> MLFTVTAPKEVYTVDVGSSVSLECDFDRRECTELEGIRASLQKVENDTSLQSERATLLEEQLPLGKALFHIPSVQVRDSGQYRCLVICGAAW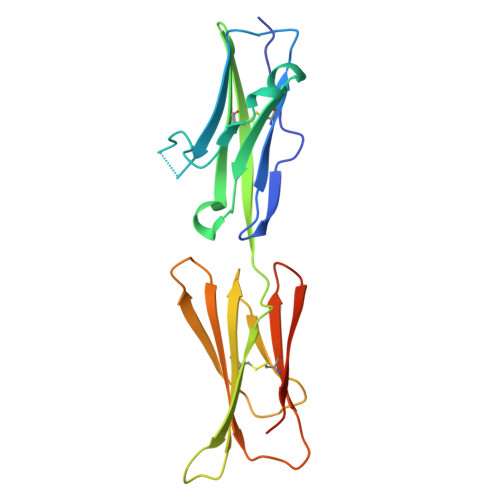DYKYLTVKVKASYMRIDTRILEVPGTGEVQLTCQARGYPLAEVSWQNVSVPANTSHIRTPEGLYQVTSVLRLKPQPSRNFSCMFWNAHMKELTSAIIDPLSRMEPKVPRT> MDKKNILPQQGQPVIRLTAGQLSSQLAELSEEALGDAGL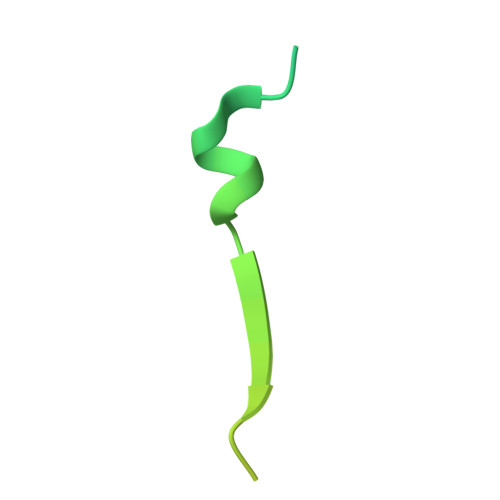EASKITACITFAAYDGELEHHHHHH>[3x]HMTHIDDYSTWDIVKATQYGIYERCRELVEAGYDVRQPDKENVTLLHWAAINNRIDLVKYYIS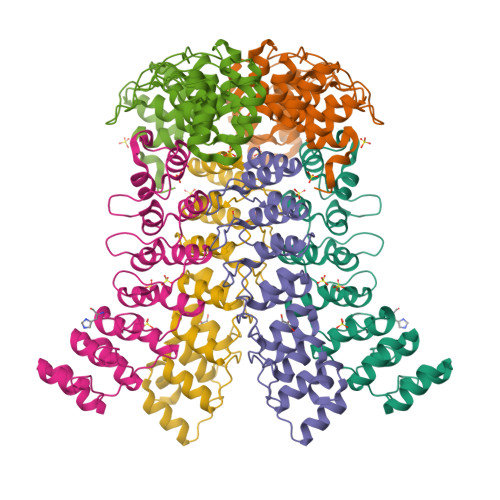KGAIVDQLGGDLNSTPLHWATRQGHLSMVVQLMKYGADPSLIDGEGCSCIHLAAQFGHTSIVAYLIAKGQDVDMMDQNGMTPLMWAAYRTHSVDPTRLLLTFNVSVNLGDKYHKNTALHWAVLAGNTTVISLLLEAGANVDAQNIKGESALDLAKQRKNVWMINHLQEARQAKGYDN> ARRVGGIGRRCFLTLHCSACSFFFQTSDAIKLILTQQHHILRKKGETRFLSGASGDAVHLESVGASNEAQGNRP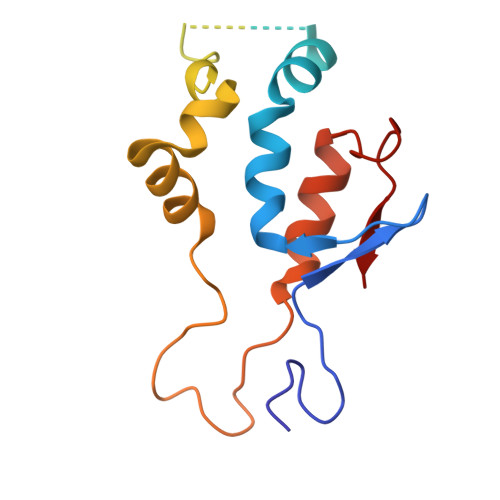SSSSSPSSSGGTRDKGVSRRVVAAAASSAASKFSLLPLADASLLLKRRGALVLRSLHGDPLVGSRRQRGEFAPQAPTAEMAKMLNKSCVPCPRCKREGRWEEG> ANIVGGIEYSINNASLCSVGFSVTRGATKGFVTAGHCGTVNATARIGGAVVGTFAARVFPGNDRAWVSLTSAQTLLPRVANGSSFVTVRGSTEAAVGAAVCRSGRTTGYQCGTITAKNITANYAEGAVRGLTQGNACMGRGDSGGSWITSAGQAQGVMSGGNVQSNGNNCGIPA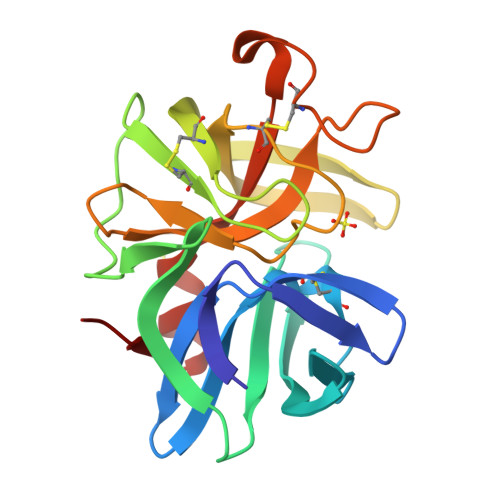SQRSSLFERLQPILSQYGLSLVTG>[2x]MTIENMSVNKSFGGWHKQYSHQSQTLNCEMRFAIYLPPQASSGKKVPVLYWLSGLTCTDENFMQKAGAQALAAELGIAIVAPDTSPRGENVADDEGYDLGKGAGFYVNATQAPWNRHYRMYDYVVDELPKLIESMFPVSDKRSIAGHSMGGHGALVIALRNADAYQSVSAFSPISNPINCPWGKKALTAYLGRDSATWMEYDASVLMRQATQFVPALVDQGDADNFLVEQLKPEVLEAAAKVKGYPLELNYREGYDHSYYFISSFIENHLRFHAEHLGK

S-formylglutathione hydrolase (SFGH, EC 3.1.2.12) is a member of the esterase family and is also known as esterase D. SFGH hydrolyzes S-formylglutathione into glutathione and formic acid and can be broadly considered an esterase, or more specifically, a thioesterase. This enzyme is involved in the glutathione-dependent formaldehyde detoxification pathway, which prevents the negative effects of formaldehyde by a series of enzymatic reactions involving formaldehyde dehydrogenase (FALDH, S-hydroxymethylglutathione dehydrogenase) and SFGH, which depend upon the spontaneous binding of glutathione to formaldehyde. Sequence alignment analyses have shown that SFGH has a conserved sequence motif (GHSMGG) that harbors catalytic serine; thus, this enzyme is also referred to as a serine hydrolase. In this study, we characterized a novel cold-active S-formylglutathione hydrolase (SfSFGH) homolog from a psychrophilic bacterium, Shewanella frigidimarina.

The crystal structure of SfSFGH was determined to a resolution of 2.32 Å using a molecular replacement method. SfSFGH was crystallized in space group P21 with two monomers in the asymmetric unit. The monomeric structure of SfSFGH includes 12 α-helices and 9 β-strands. The conserved catalytic triad residues of Ser148, Asp224, and His257 are located in this groove. The catalytic residue Ser148 is located in the short β6-α6 loop region and directly interacts with His257 located in the β9-α12 loop region. In addition, the oxyanion hole comprising the backbone amides Leu55 and Met149 can be observed at the neighboring active site. In the apo state of the SfSFGH structure, oxyanion holes are occupied by water molecules. The vicinity of the substrate-binding site is positively charged by the Lys65 and His147. Especially, the β5-α4 loop region (residues 83–112) in SfSFGH has a significantly different conformation with a relatively higher main chain B-factor value (27.9 Å2) than overall B-factor value (24.7 Å2). Our sequence alignment results also show that only cold-active enzymes have a conserved glycine residue in this β5-α4 loop region (Gly96 in SfSFGH and Gly96 in OLEI01171). Collectively, it is thought that the flexibility of the β5-α4 loop region and the open active site are related to the cold-activity of SfSFGH.> CC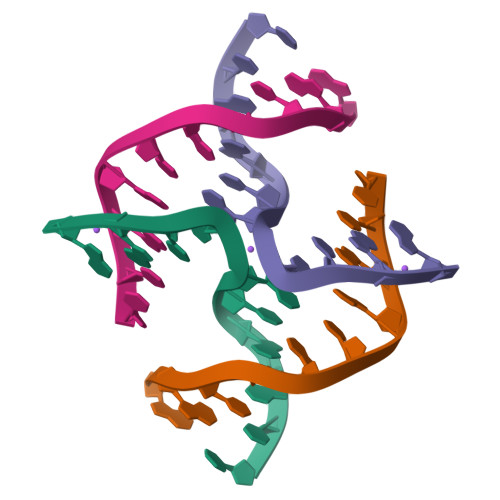GATACCGG;> CCGGTAUCGG> MAITVKGLTNKLTRTQRRIAVVEFIFSLLFFL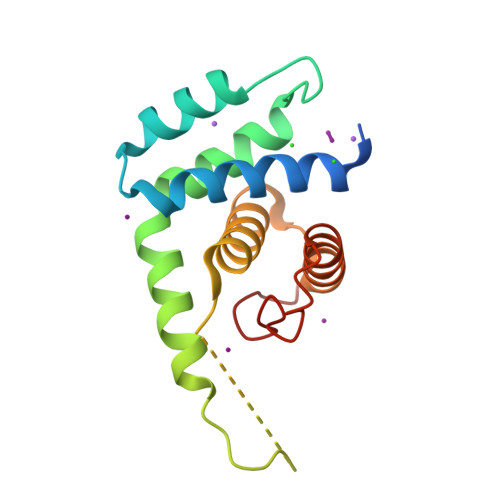PKEAEVIQADFLEYDTKERQLNEWQKLIVKAFSENIFSFQKKIEEQQLKNQLEIQTKYNKISGKKIDLLTTAVVLCALSEQKAHNTDKPLLISEALLIMDHYSQGAEKKQTHALLDKLL> MNTQSLMSSTHTIAASDPHIQVMGRTHINDDASLTFGYPGVSLSTIVAGSRLTAEMQSSNGNSWIDVIIDNHPPTSIKLDAQQQTVELFHFPNSGEHRVEIIHRSENWHGQVTLKQLTLTGTQFLPAPVLPQRKILVLGDSVTCGEAIDRVAGEDKNTRWWNARESYGMLTAKALDAQVQLVCWGGRGLIRSWNGKTDDANLPDFYQFTLGDTG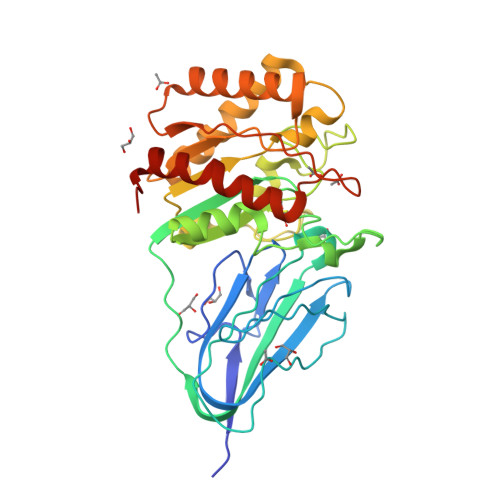QAPQWDHHRYQPDLIISAIGTNDFSPGIPDRATYINTYTRFVRTLLDNHPQATIVLTEGAILNGDKKAALVSYIGETRQQLHSNRVFYASSSHHPGDNSDAHPTKDQHAAMARELTPQLRQIMDWLEHHHHHH> LGSMVATVKRTIRIKTQQHILPEVPPVENFPVRQWSIEIVLLDDEGKEIPATIFDKVIYHLHPTFANPNRTFTDPPFRIEEQGWGGF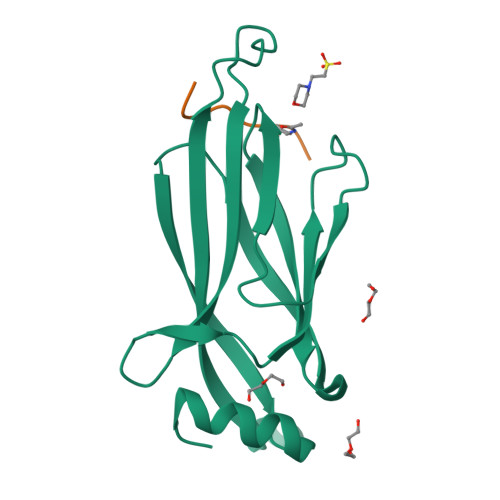PLDISVFLLEKAGERKIPHDLNFLQESYEVEHVIQIPLNKPLLTEELAKSGST;> AQTARKST> MPPNSATRWLPFVSSDLKDYLNRYWAVMF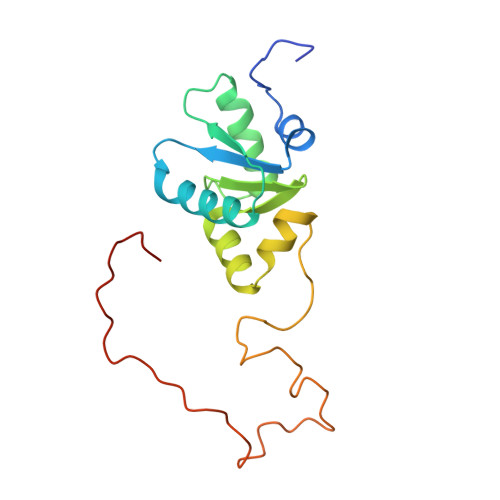TVGARPIETGHIRHYVSWYCTRMKVVLLDHHVYVEPLRQQLQEASRTPELPLLFVNKKLVGTLRDVELLEREKKLKDVLHFGFEWRVGGSVAATNGQKSLMGALPAPYGDAEFFRGRYRGPPVARPVVSLPTLHPFALRSEE Phage satellite P4 polarity suppression protein, Psu, a building block of the viral capsid, inhibits hexameric transcription termination factor, ρ, by presently unknown mechanisms. The ρ hexamer adopts an NTPase-inactive, washer-like, open-ring conformation until NTPs (preferentially ATP) are engaged and RNA is bound at the SBS, leading to ring closure and RNA entrapment inside the ring. Our cryogenic electron microscopy structures of ρ-Psu complexes show that Psu dimers clamp two inactive, open ρ rings and promote their expansion to higher-oligomeric states. ATPase, nucleotide binding and nucleic acid binding studies revealed that Psu hinders ρ ring closure and traps nucleotides in their binding pockets on ρ.

Irrespective of the bound nucleotide, all assemblies contain two open ρ rings, denominated ρ(A) and ρ(B), that are laterally bridged by multiple Psu dimers, with the ρ CTDs facing inwards and the ρ NTDs facing outwards. In complex II, two hexameric ρ rings are bridged by five Psu dimers that connect ρ(A) subunit 6 with ρ(B) subunit 2, ρ(A) subunit 5 with ρ(B) subunit 3, etc. The different rotational orientations of the Psu-bridged ρ rings in complexes I, II, and III lead to different spacings between the innermost ρ subunits, which directly interact in complex I but are separated by a gap of ~ 30 Å and ~50 Å in complexes II and III, respectively. We further refined complex II (ATP; global resolution 3.8 Å), complex IIexpanded (ATP; global resolution 3.6 Å), complex III (ATPγS; global resolution 3.65 Å), and complex IIIexpanded (ATPγS; global resolution 4.25 Å). The ρ hexamers in complexes I, II and III exhibit slightly increased inter-subunit and ρ1-ρ6 rise values (8.4–8.8 Å and 42.2–43.9 Å, respectively). Psu subunits bind between two neighboring ρ CTDs across the nucleotide-binding sites. Psu helix α7 (residues 170–186) is placed in a cleft between the two neighboring ρ CTDs, covering the corresponding nucleotide-binding pocket. ATP or ATPγS are bound similarly between all neighboring ρ CTDs in the ρ-ATP/ATPγS-Psu or ρP167L-ATPγS-Psu assemblies.

>[12x]MNLTELKNTPVSELITLGENMGLENLARMRKQDIIFAILKQHAKSGEDIFGDGVLEILQDGFGFLRSADSSYLAGPDDIYVSPSQIRRFNLRTGDTISGKIRPPKEGERYFALLKVNEVNFDKPENARNKILFENLTPLHANSRLRMERGNGSTEDLTARVLDLASPIGRGQRGLIVAPPKAGKTMLLQNIAQSIAYNHPDCVLMVLLIDERPEEVTEMQRLVKGEVVASTFDEPASRHVQVAEMVIEKAKRLVEHKKDVIILLDSITRLARAYNTVVPASGKVLTGGVDANALHRPKRFFGAARNVEEGGSLTIIATALIDTGSKMDEVIYEEFKGTGNMELHLSRKIAEKRVFPAIDYNRSGTRKEELLTTQEELQKMWILRKIIHPMGEIDAMEFLINKLAMTKTNDDFFEMMKRS;>[10x]MESTALQQAFDTCQNNKAAWLQRKNELAAAEQEYLRLLSGEGRNVSRLDELRNIIEVRKWQVNQAAGRYIRSHEAVQHISIRDRLNDFMQQHGTALAAALAPELMGYSELTAIARNCAIQRATDALREALLSWLAKGEKINYSAQDSDILTTIGFRPDVASVDDSREKFTPAQNMIFSRKSAQLASRQSV> MEEPEEPADSGQSLVPVYIYSPEYVSMCDSLAKIPKRASMVHSLIEAYALHKQMRIVKPKVASMEEMATFHTDAYLQHLQKVSQEGDDDHPDSIEYGLGYLCPATEGIFDYAAAIGGATITAAQCLIDGMCKVAINWSGGW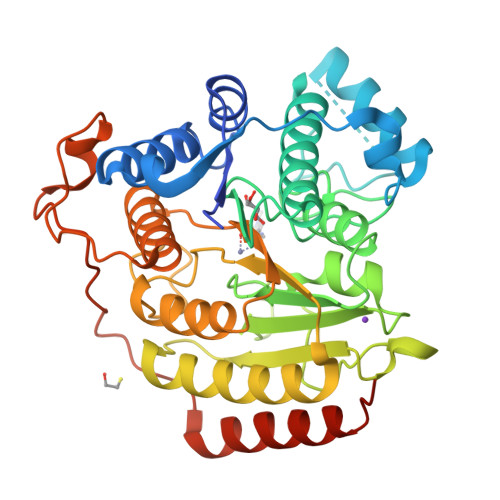HHAKKDEASGFCYLNDAVLGILRLRRKFERILYVDLDLHHGDGVEDAFSFTSKVMTVSLHKFSPGFFPGTGDVSDVGLGKGRYYSVNVPIQDGIQDEKYYQICESVLKEVYQAFNPKAVVLQLGADTIAGDPMCSFNMTPVGIGKCLKYILQWQLATLILGGGGYNLANTARCWTYLTGVILGKTLSSEIPDHEFFTAYGPDYVLEITPSCRPDRNEPHRIQQILNYIKGNLKHVVIEGRSHHHHHH> MQTQEVAIKPNLKVVLRSDAQQIDEVVVTAMGIKRSEKALGYAATSVGGEKIAESRTSDVMSSLAGKIAGVQISSTSSDPGASNSVIIRGVSSLSGTNQPLYVVDGVPLNNSTVYSTDGLNSGYDFGNGANAINPDDVANMTILKGAAATALYGSRAANGVVMITTKSGRKEKGVGIEYNGGVQWSTVLRLPEFQNEFGMGWNGNHTELENGSWGPRFDGSMQLWGNVYNNSQKLKPYVAMPDNIKDFFDAGFRYSNSLSFNGATDKSDYYVSFSQISDDGMIPTDADSYDKYTFSARGSHKAGALTFSSSLNYAYQKNNFATTGQGLSMLNSLYQTPRDISIIGLEDQNDPFNTPGYYYTPYGVMNPYYILNNYLNEYESERFYGKFQLDYEFLKYFKFTYRMGLDTTTGQSDKGKPNLYALYYEGTPNGEGQGSSSPFSGETGQYSEQITRRREINQDIMVNFNMPVNDFNINALVG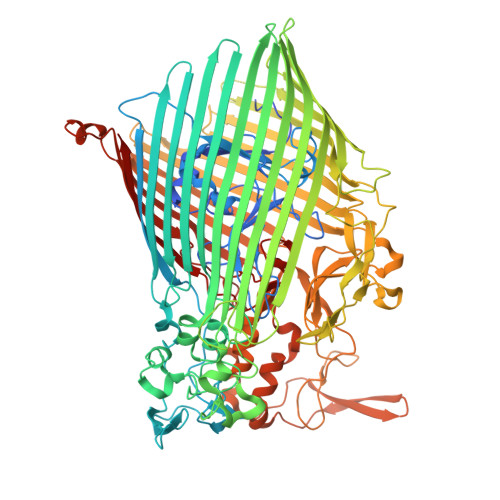FNGNERKVSYQYSEVNDLTIPTWFNLKNSGKTPIVEQHMELRRLMGVFGQFEGSWKNMLYLTVTARNDWSSTLPKENRSFFYPGITGSFIFSELLNDNLQDVITFGKIRASWGKTGNDADVYMVNPVYAQSSNRIPFGSLTFPLGGVNAYSAGNVLGSNTLSPEMTTESEVGLNMAFFKNRLSFDVSYYNRNTDKQIFSLAMDPASGYTAQNMNLGKIRNRGIELLISGTPIRTKDFSWELTWNFTKNWSKVISLPEELGGITTIYGLNGGTSMYAITGMPVGVFKAQVAERDPQGRIVVNSSTGLPVEASEFGICGDMNNKYQMGVSTNLKYKGISLGIDFDIRQGGVMYSRTKDINYFTGNAIQTAYNDRNPLIVPNSVNKIVNGENVTYVENTTPITSSNIYKYWGDGGSDMGSCFLVDKSYVKLRSVVLGWDLPKRWLAKTPFQAVKVSAYGNNLFVWTPSSNTFIDPEMTSFGNDLEGNYGEYTANPSSRRFGFNLMVKF>VQDCYHGDGQSYRGTSSTTTTGKKCQSWSSMTPHRHQKTPENYPNAGLTMNYCRNPDADKGPWCFTTDPSVRWEYCNLKKCSGTEAS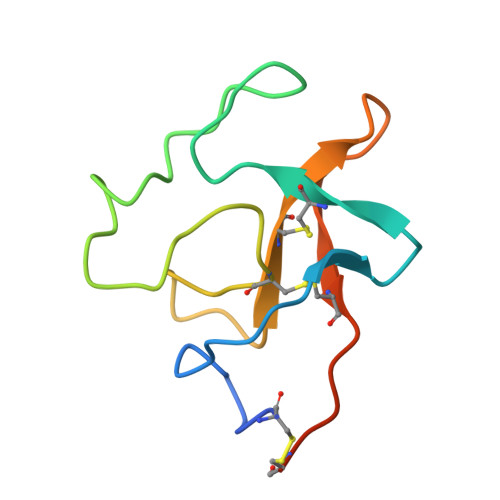V[2x]(2Z)-2-iminopentanedioic 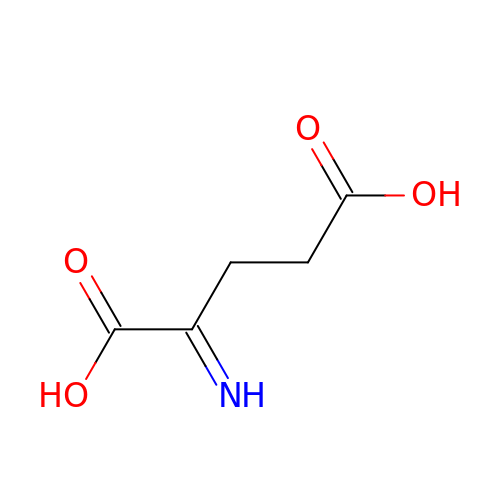acid | C5 H7 N O4 | UZWLXPOZNAJCJV-UTCJRWHESA-N> GAMADTCMSRIVKEYKVILKTLASDDPIANPYRGIIESLNPIDETDLSKWEAIISGPSDTPYENHQFRILIEVPSSYPMNPPKISFMQNNILHSNVKS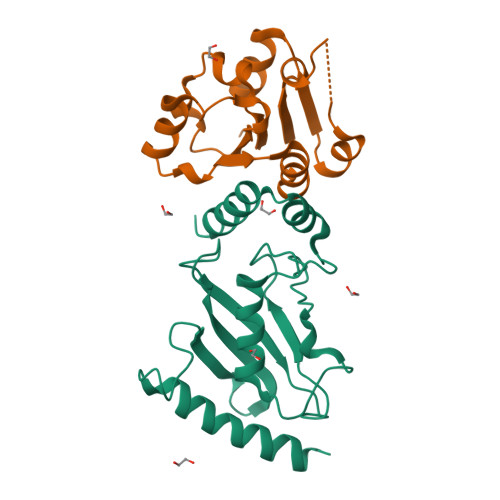ATGEICLNILKPEEWTPVWDLLHCVHAVWRLLREPVSDSPLDVDIGNIIRCGDMSAYQGIVKYFLAERERINNH;> GAMENKKARKSKCIIMSKSIQGLPIKWEEYAADEVVLLVPTSHTDGSMKQAIGDAFRKTKNEHKIIYCDSMDGLWSCVRRLGKFQCILNSRDFTSSGGSDAAVVPEDIGRFVKFVVDSDVEDVLIDTLCN> ETSYTLNEVVPL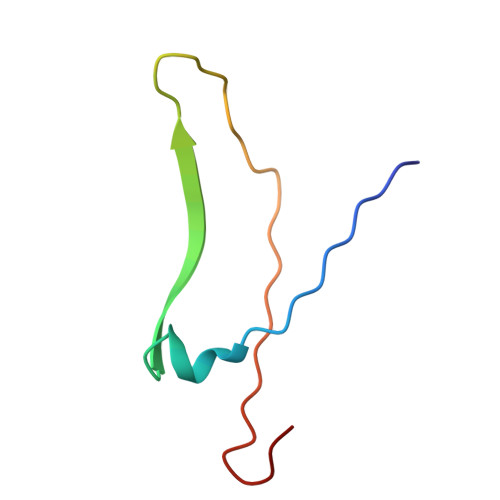KEFVPEWVRIGFSATTGAEFAAHEVLSWYFHSELAGTSSN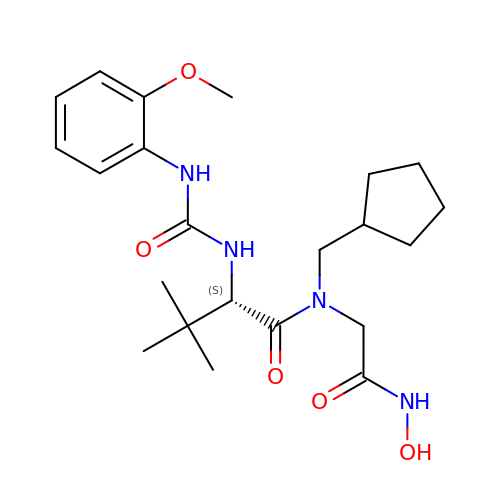(S)-N-(cyclopentylmethyl)-N-(2-(hydroxyamino)-2-oxoethyl)-2-(3-(2-methoxyphenyl)ureido)-3,3-dimethylbutanamide | C22 H34 N4 O5 | SGGVRJBZDBEGBH-LJQANCHMSA-N> MASSRRESINPWTLTGFADAEGSFGLSILNRNRGTARYHTRLSFTIMLHNKDKSILENIQSTWKVGSILNNGDHYVSLVVYRFEDLKVIIDHFEKYPLITQKLGDYKLFKQAFSVMENKEHLKENGIKELVRIKAKMNWGLNDELKKAFPEVIS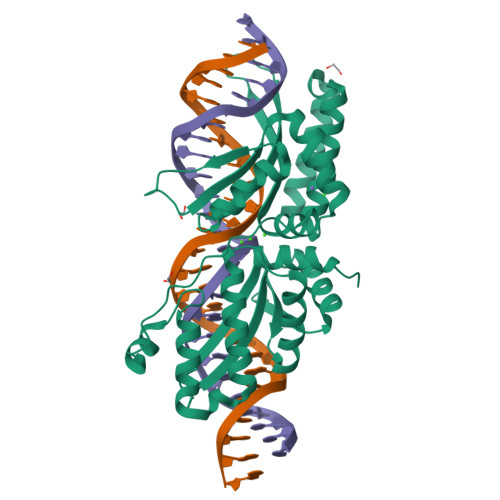RERPLINKNIPNGKWLAGFTSGDGSFFVRLRKSNVNARVRVQLVFEISQHIRDKNLMNSLITYLGCGHIYEGNKSERSWLQFRVEKFSDINDKIIPVFQENTLIGMKLEDFEDWCKVAKLIEEKKHLTESGLDEIKKIKLNMNKRR> GSHMKNLLRAINPLNRPQTERLDERQVRNNAGGFVYTVSDESRLTRFLVLGVDGGTFYASAQKHTVQATDFVRELVQR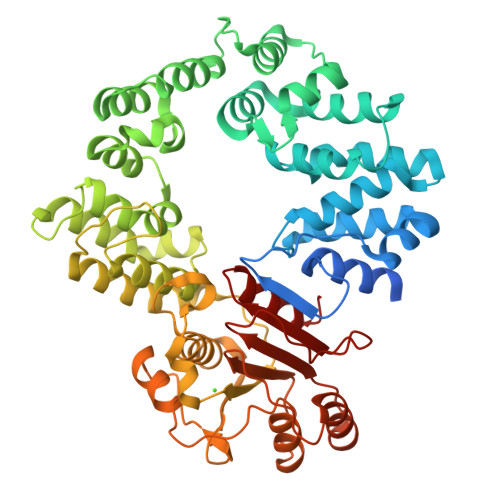DAALALRVTLDVVRGQRAPKADPALLVLALIAKTAPNAADRKAAWDALPEVARTGTMLLHFLAFADALGGWGRLTRRGVANVYETADVDKLALWAVKYKARDGWSQADALRKAHPKTDDAARNAVLKFMVDGVLPKVDSPALRVIEGHLKATEAQTDAAAAALMQEYRLPLEAVPTHVRGAEVYRAAMQTNGLTWLLRNLGNLGRVGVLTPNDSATVQAVIERLTDPAALKRGRIHPLDALKARLVYAQGQGVRGKGTWLPVPRVVDALEEAFTLAFGNVQPANTRHLLALDVSGSMTCGDVAGVPGLTPNMAAAAMSLIALRTEPDALTMGFAEQFRPLGITPRDTLESAMQKAQSVSFGGTDCAQPILWAAQERLDVDTFVVYTDNETWAGQVHPTVALDQYAQKMGRAPKLIVVGLTATEFSIADPQRRDMLDVVGFDAAAPNVMTAFARGEVL Clostridium histolyticum collagenases ColG and ColH are segmental enzymes that are thought to be activated by Ca2+-triggered domain reorientation to cause extensive tissue destruction. The collagenases consist of a collagenase module (s1), a variable number of polycystic kidney disease-like (PKD-like) domains (s2a and s2b in ColH and s2 in ColG) and a variable number of collagen-binding domains (s3 in ColH and s3a and s3b in ColG). The X-ray crystal structures of Ca2+-bound holo s2a (space group C2), Ca2+-free apo s2a (space group P61), Ca2+-bound holo s2b (space group P21) and two new forms of N-terminally truncated wild-type apo s2 (space groups P21 and P212121) are reported for the first time. Comparison of crystal structures of ColG s2 with crystal structures of ColH s2a and s2b suggests that despite common tertiary folds, PKD-like domains can be grouped into two subsets.

Of the novel s2a and s2b structures, that of s2b was solved at higher resolution and therefore is described in the most detail. Similar to holo s2a, the two NCS-related holo s2b structures are virtually identical (r.m.s.d. of 0.4 Å). Each holo s2b structure begins at residue 766 and the last residue is 860. The first bulge occurs when Pro784 breaks β-strand A and pushes the subsequent Lys785 outwards, which in turn leads to an approximately 127° angle between β-strands A and A′ that also changes the allegiance of β-strand A′ to β-strand G. The second conserved bulge is introduced by Lys798 and Gly799. Temperature factors for both NCS-related structures are low (the average B factor for molecule A is 11.7 Å2 and that for molecule B is 9.9 Å2). Anisotropic B-factor analyses using the Anisotropic Network Model (ANM) web server showed that the main chain is mostly isotropic and that potential correlated movement occurs exclusively at the N-terminal linker. In s2b, the insertion of Asp819 results in the region adopting an ω-loop (i→i + 10). In s2b, Ca2+ chelation by Asn774 and Lys775 could stabilize a 310-helix (residues 770–774) that aligns with the cylinder axis. Meanwhile, the N-terminal linker structure of a PKD-like domain is described for the first time in the holo s2b structure and suggests that Ca2+ repositions the linker along the barrel axis. Of the three domains, s2b is the most stable.

>[2x]AEIKDLSENKLPVIYMHVPKSGALNQKVVFYGKGTYDPDGSIAGYQWDFGDGSDFSSEQNPSHVYTKKGEYTVTLRVMDSSGQMSEKTMKIKITD> ATSVVAWGGNNDWGEATVPAEAQSGVDAIAGGYFHGLALKGGKVLGWG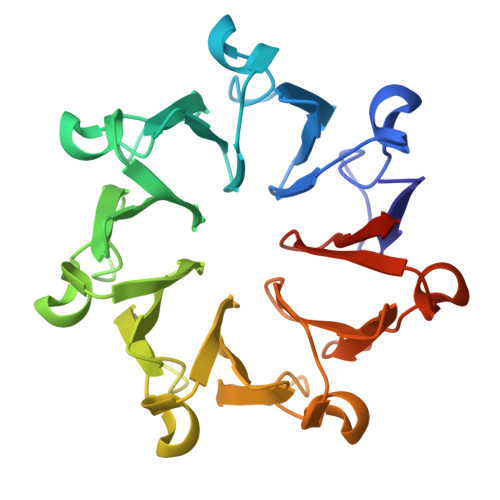ANLNGQLTMPAATQSGVDAIAAGNYHSLALKDGEVIAWGGNEDGQTTVPAEARSGVDAIAAGAWASYALKDGKVIAWGDDSDGQTTVPAEAQSGVTALDGGVYTALAVKNGGVIAWGDNYFGQTTVPAEAQSGVDDVAGGIFHSLALKDGKVIAWGDNRYKQTTVPTEALSGVSAIASGEWYSLALKNGKVIAWGSSRTAPSSVQSGVSSIEAGPNAAYALKGGSGSGHHHHHH> NIPFTNNLLFSGQVLYGDGRLTAKNHQLVMQGDCNLVLYGGKYGWQSNTHGNGEHCFLRLNHKGELIIKDDDFKTIWSSSSSSKQGDYVL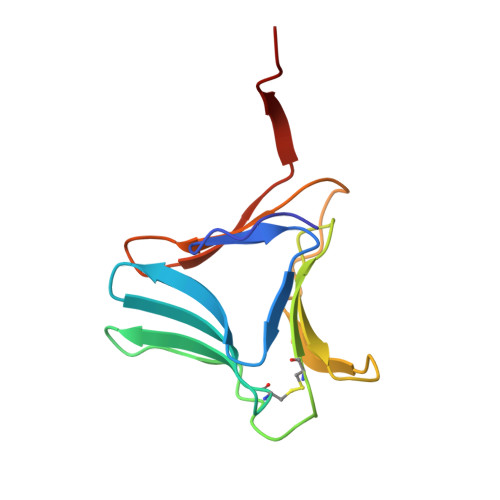ILRDDGFAVIYGPAIWETSPQ>[3x]METLFSGIQPSGIPTIGNYIGALKQFVDVQNDYDCYFCIVDQHAITMPQDRLKLRKQTRQLAAIYLASGIDPDKATLFIQSEVPAHVQAGWMLTTIASVGELERMTQYKDKAQKAVEGIP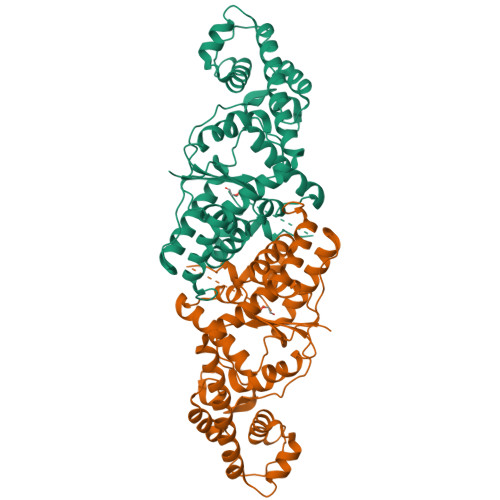AGLLTYPPLMAADIVLYNTNIVPVGDDQKQHIELTRNLVDRFNSRYNDVLVKPEIRMPKVGGRVMSLQDPTRKMSKSDDNAKNFISLLDEPNVAAKKIKSAVTDSDGIIKFDRDNKPGITNLISIYAGLTDMPIKDIEAKYEGEGYGKFKGDLAEIVKAFLVEFQEKYESFYNSDKLDDILDQGRDKAHKVSFKTVKKMEKAMGLGRKRHHHHHH> MPKTQAEILTLDFNLAELPSAQHRAGLAGLILMIRELKKWPWFKIRQKEKDVLLSIENLDQYGASIQLNLEGLIALFDLAYLSFTEERKSKSKIKDFKRVDEIEIEENGKNKIQKYYFYDVITPQGGFLAGWDKSDGQIWLRIWRDMFWSIIKGVPATRNPFNNRCGLNLNAGDSFSKDVESVWKSLQNAEKTTGQSGAFYLGAMAVNAENVSTDDLIKWQFLLHFWAFVAQVYCPYILDKDGKRNFNGYVIVIPDIANLEDFCDIL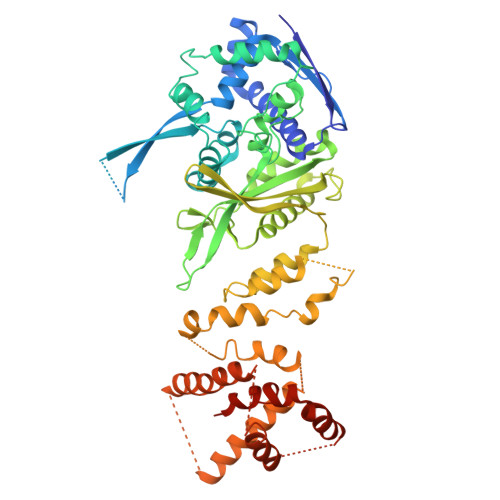PDVLSNRNSKAFGFRPQESVIDVPEQGALELLNLIKQRIAKKAGSGLLSDLIVGVEVIHAEKQGNSIKLHSVSYLQPNEESVDDYNAIKNSYYCPWFRRQLLLNLVNPKFDLASQSWLKRHPWYGFGDLLSRIPQRWLKENNSYFSHDARQLFTQKGDFDMTVATTKTREYAEIVYKIAQGFVLSKLSSKHDLQWSKCKGNPKLEREYNDKKEKVVNEAFLAIRSRTEKQAFIDYFVSTLYPHVRQDEFVDFAQKLFQDTDEIRSLTLLALSSQYPIKRQGETE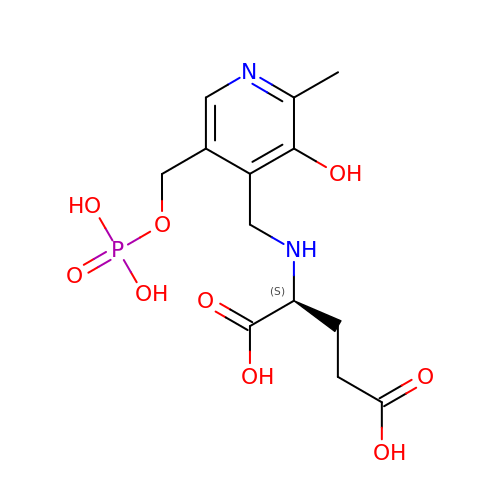N-({3-hydroxy-2-methyl-5-[(phosphonooxy)methyl]pyridin-4-yl}methyl)-L-glutamic acid | C13 H19 N2 O9 P | JMRKOGDJNHPMHS-JTQLQIEISA-N>[4x]MKTYNVDENGYYGEFGGAYIPEILHKCVEDLQNNYLKILESPDFQKEYDQLLRDYVGRPSPLYLAKRLSEKYGCKIYLKREDLNHTGAHKINNTIGQILLARRMGKTRIIAETGAGQHGVATA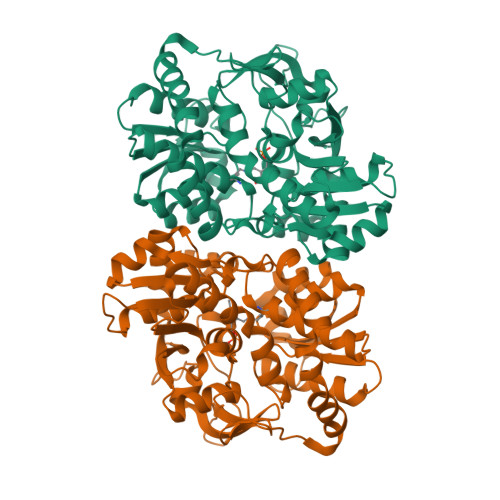TVCALMNMECIVYMGKTDVERQHVNVQKMEMLGATVVPVTSGNMTLKDATNEAIRDWCCHPSDTYYIIGSTVGPHPYPDMVARLQSVISKEIKKQLQEKEGRDYPDYLIACVGGGSNAAGTIYHYIDDERVKIVLAEAGGKGIDSGMTAATIHLGKMGIIHGSKTLVMQNEDGQIEEPYSISAGLDYPGIGPMHANLAKQKRAQVLAINDDEALNAAFELTRLEGIIPALESAHALAALEKVKFKPEDVVVLTLSGRGDKDMETYLKYKKNSNE> EDERIVLVDNKCKCARITSRIIRSSEDPNEDIVERNIRIIVPLNNRENISDPTSPLRTRFVYHLSDLCKKCDPTEVELDNQIVTATQSNICDEDSATETCY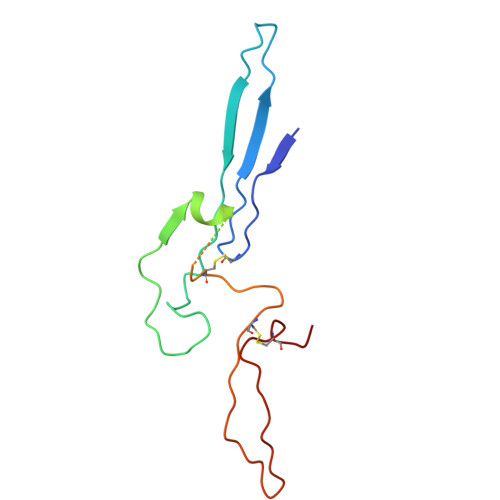TYDRNKCYTAVVPLVYGGETKMVETALTPDACYPD>ACTWPAWEQFKKDYISQEGRVIDPSDARKITTSEGQSYGMFSALAANDRAAFDNILDWTQNNLAQGSLKERLPAWLWGKKENSKWEVLDSNSASDGDVWMAWSLLEAGRLWKEQRYTDIGSALLKRIAREEVVTVPGLGSMLLPGKVGFAEDNSWRFNPSYLPPTLAQYFTRFGAPWTTLRETNQRLLLETAPKGFSPDWVRYEKDKGWQLKAEKTLISSYDAIRVYMWVGMMPDSDPQKARMLNRFKPMATFTEKNGYPPE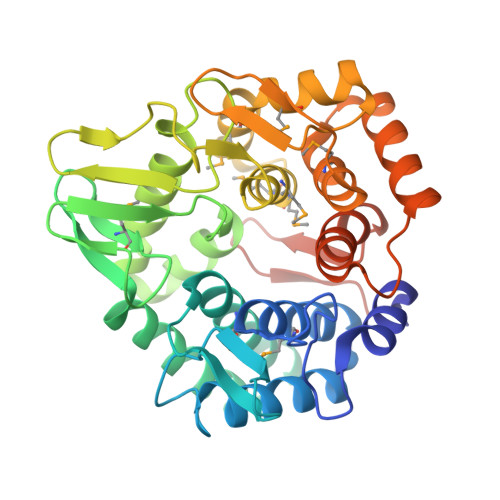KVDVATGKAQGKGPVGFSAAMLPFLQNRDAQAVQRQRVADNFPGSDAYYNYVLTLFGQGWDQHRFRFSTKGELLPDWGQECANSHLEHHHHHH[4x]>DEITKKYIKDNIINVDDNIIKKKDIFKLKNENNEITECAFEYFESKKKFDDDIESRFFIINDNNYNENINLIYKDIKYCGLNIQTTGLEVFDENIRLIQIAVENYPVIIYDMFNINKKDILDGLRKVLENKNIIKIIQNGKFDAKFLLHNNFKIENIFDTYIASKLLDKNKNMYGFKLNNIVEKYLNVILDKQQQNSVWNNSLLNNNQLFYAARDSSCLLKLYKKLKEEIKKENLHIVNDIENKCILPICDMELNGIKVDLENLQKSTNEILNELNIEKDNLKKKLKDENINVNSQQQVLKALQKNNVRDISNKLIENTSDSNLKNFLNHEEIISLRNYRRL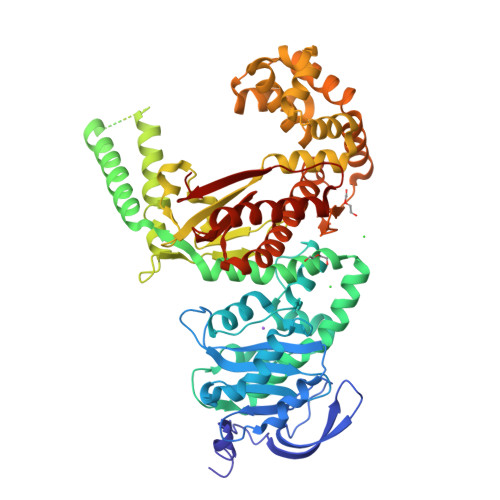YKLYSAFYLKLPLHINTKTNKIHTTFNQLKTFSGRFSSEKPNLQQIPRQKNIREIFIPNDNNIFIIADFKQIELKIAAEITNDEIMLKAYNNNIDLHTLTASIITKKNIPDINKEDRHIAKAINFGLIYGMNYVNLKNYANTYYGLNMSLDQCLYFYNSFFEHYKGIYKFHNQVKQKRALQYSTLSNRKVIFPYFSFTKALNYPVQGTCADILKLALVDLYDNLKDINGKIILCVHDEIIIEVNKKFQEEALKILVQSMENSASYFLKKVKCEVSVKIAENWGSKD[2x]>[4x]ADPGGSHHHHH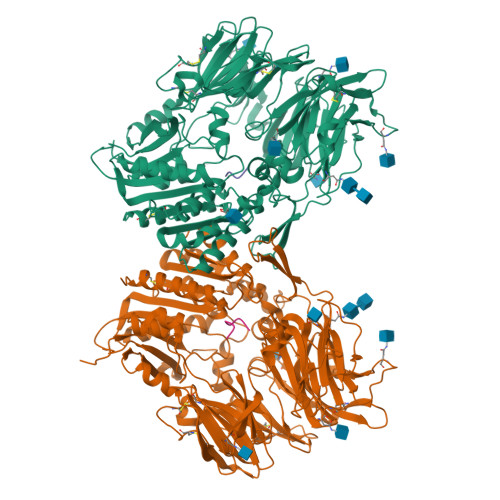SRKTYTLTDYLKNTYRLKLYSLRWISDHEYLYKQENNILVFNAEYGNSSVFLENSTFDEFGHSINDYSISPDGQFILLEYNYVKQWRHSYTASYDIYDLNKRQLITEERIPNNTQWVTWSPVGHKLAYVWNNDIYVKIEPNLPSYRITWTGKEDIIYNGITDWVYEEEVFSAYSALWWSPNGTFLAYAQFNDTEVPLIEYSFYSDESLQYPKTVRVPYPKAGAVNPTVKFFVVNTDSLSSVTNATSIQITAPASMLIGDHYLCDVTWATQERISLQWLRRIQNYSVMDICDYDESSGRWNCLVARQHIEMSTTGWVGRFRPSEPHFTLDGNSFYKIISNEEGYRHICYFQIDKKDCTFITKGTWEVIGIEALTSDYLYYISNEYKGMPGGRNLYKIQLSDYTKVTCLSCELNPERCQYYSVSFSKEAKYYQLRCSGPGLPLYTLHSSVNDKGLRVLEDNSALDKMLQNVQMPSKKLDFIILNETKFWYQMILPPHFDKSKKYPLLLDVYAGPCSQKADTVFRLNWATYLASTENIIVASFDGRGSGYQGDKIMHAINRRLGTFEVEDQIEAARQFSKMGFVDNKRIAIWGWSYGGYVTSMVLGSGSGVFKCGIAVAPVSRWEYYDSVYTERYMGLPTPEDNLDHYRNSTVMSRAENFKQVEYLLIHGTADDNVHFQQSAQISKALVDVGVDFQAMWYTDEDHGIASSTAHQHIYTHMSHFIKQCFSLP;>YPSKPDNPGE[4x]> FGNKYIQQTKPLTLERTINLYPLTNYTFGTKEPLYEKDSSVAARFQRMREEFDKIGMRRTVEGVLIVHEHRLPHVLLLQLGTTFFKLPGGELNPGEDE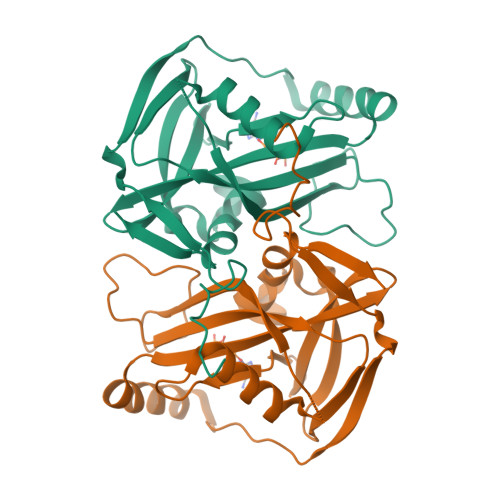VEGLKRLMTEILGRQDGVLQDWVIDDCIGNWWRPNFEPPQYPYIPAHITKPKEHKKLFLVQLQEKALFAVPKNYKLVAAPLFELYDNAPGYGPIISSLPQLLSRFNFIYN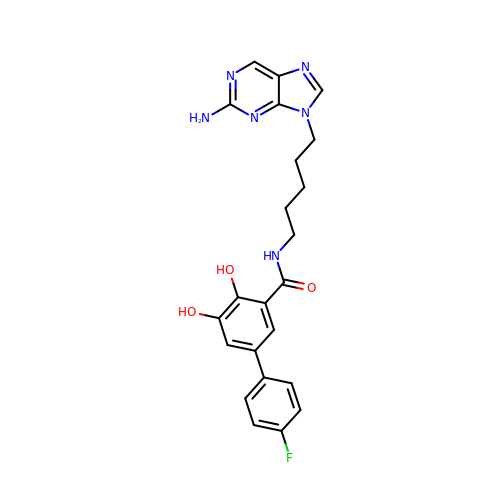N-[5-(2-aminopurin-9-yl)pentyl]-5-(4-fluorophenyl)-2,3-dihydroxybenzamide | C23 H23 F N6 O3 | KUZQYEZWVYHXLQ-UHFFFAOYSA-N> QAVQPVDFRHHHFSDMEIFLRRYANEYPSITRLYSVGKSVELRELYVMEISDNPGIHEAGEPEFKYIGNMHGNEVVGRELLLNLIEYLCKNFGTDPEVTDLVQSTRIHIMPSMNPDGYEKSQEGDRGGTVGRNNSNNYDLNRNFPDQFFQVTDPPQPETLAVMSWLKTYPFVLSANLHGGSLVVNYPFDDDEQGIAIYSKSPDDAVFQQLALSYSKENKKMYQGSPCKDLYPTEYFPHGITNGAQWYNVPGGMQDWNYLNTNCFEVTIE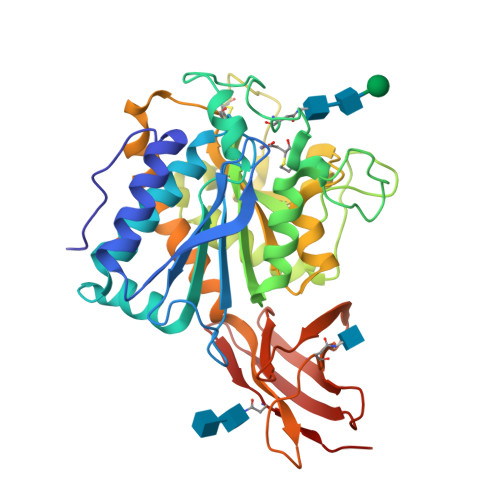LGCVKYPKAEELPKYWEQNRRSLLQFIKQVHRGIWGFVLDATDGRGILNATISVADINHPVTTYKDGDYWRLLVQGTYKVTASARGYDPVTKTVEVDSKGGVQVNFTLSRT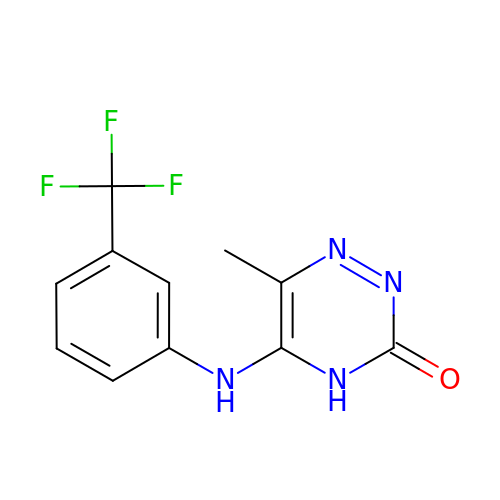6-methyl-5-{[3-(trifluoromethyl)phenyl]amino}-1,2,4-triazin-3(4H)-one | C11 H9 F3 N4 O | DDMOHNSTFUBVJB-UHFFFAOYSA-N> MIKQFLLGVASILPLFSAPALSDSLPERIDTFTELFNYEVALKSYDIRILQSNYPTKLLSPDSLLPQTSDYPLKDIQQLYSLANTCRGKLPLSPLITEPLVFTRAICKGTQLTPRWFSRSGLIHPGGGTYAARYVEKYPELRPKLAQYMHIKERDNEEGDELLESLQNMDDD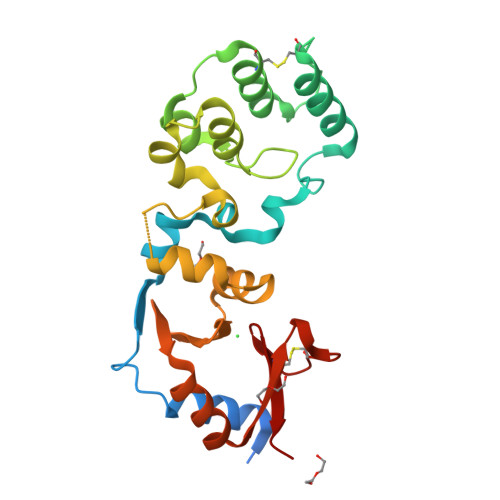AINALIAGASMFIEGKEMWLRRGDRYFVFSKDVWQENVANAGLSYTLASQSKSCFVKRGNICWDVEDH>HMTFKAEYIWIDGTEPTAKLRSKTKIITAAPAGLDALPVWGFDGSSTNQAEGSSSDCVLKPVFSCPDPIRGGEDILVLCEVLDTDMTPHPSNTRAALAELSERFAAQEPVFGIEQEYTFFKGTRPLGFPEGGFPAAQGGYYCGVGSDEIFGRDVVEAHLENCLKAGLGISGINAEVMPGQWEFQVGPLAPLEVSDQLWVARWLLYRTAEDFEVSATLDPKPVKGDWNGAGAHTNFSTKAMREGYDAIITAAESLGEGSKPMDHVKNYGAGIDDRLTGLHETAPWN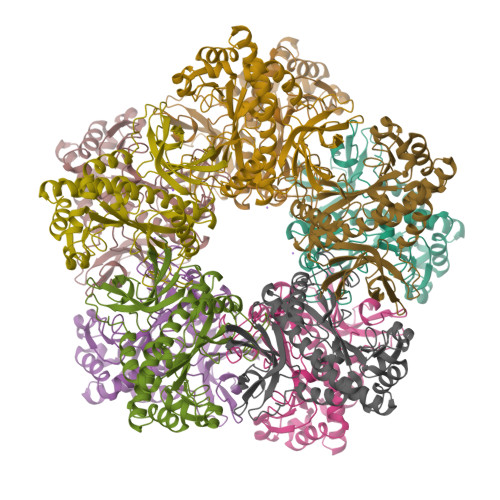EYSYGVSDRGASVRIPWQVEKDGKGYIEDRRPNANVDPYVVTRLLVDTCCTALEKAGQV[10x]>[2x]PLGSGVPKEIQLAELREALLGIPGVTGLHDLHVWSITSGKISLTS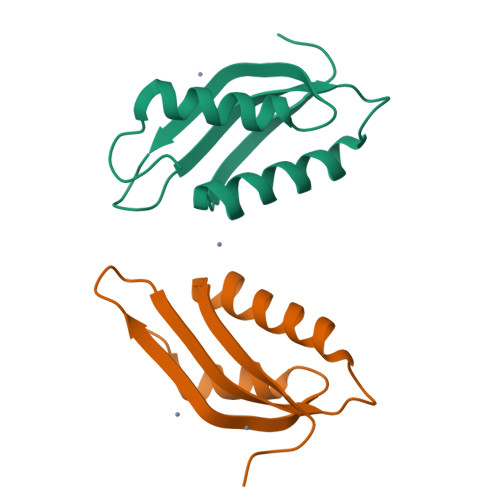HLVYDPALVDAEALLGTVKALLHDRYEIEHSTLQLETSACA> MVKVGGEAGPSVTLPCHYSGAVTSMCWNRGSCSLFTCQNGIVWTNGTHVTYRKDTRYKLLGDLS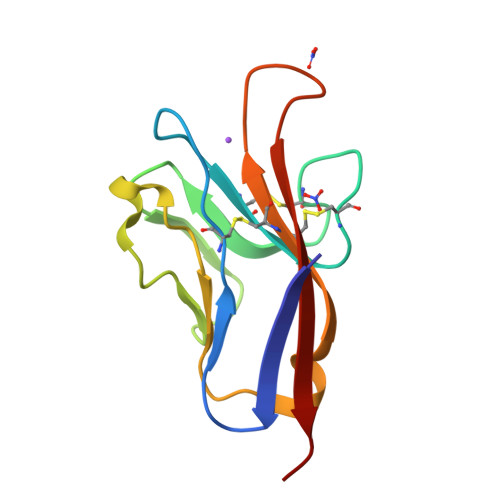RRDVSLTIENTAVSDSGVYCCRVEHRGWFNDMKITVSLEIVPP> HMPREPVTPDSDHPDPVETVRQLTAHVLGLTAAADVEM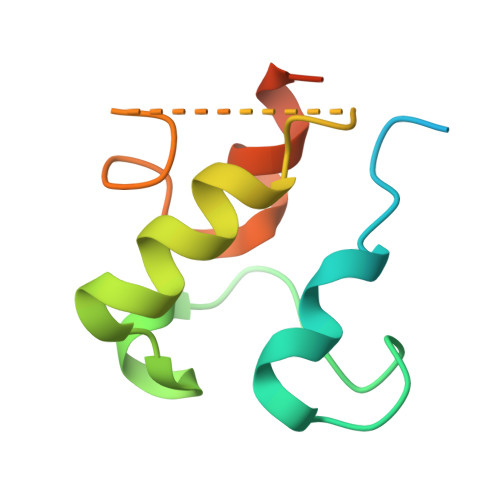TRSFKDLGFDSLMSVELRDRLCAATGLSLATTLLYDHPSPAETAEFVRARLTGDEA However, exceptionally high-level aminoglycoside-resistance is achieved by the action of intrinsic and acquired 16S ribosomal RNA (rRNA) methyltransferase enzymes in aminoglycoside-producing and human pathogenic bacteria, respectively. These resistance determinants block drug binding by catalyzing the transfer of a methyl group from their cosubstrate S-adenosyl-l-methionine (SAM) to the base of a defined target RNA nucleotide within the ribosomal A-site. Here, we describe detailed structural and functional analyses of one of these enzymes, the kanamycin-resistance methyltransferase from Catenulisporales acidiphilia (‘CacKam’). CacKam has a SAM-binding core fold comprised of a seven-stranded β-sheet with a central topological switch point, characteristic of Class I methyltransferases.

We next exploited the altered crystal packing and constraints on the β6/7 linker in the CacKam-W203A crystal form to obtain a complex structure by soaking preformed crystals with SAM. In contrast to the apo structure of CacKam-W203A, SAM binding allowed the peptide backbone path of the β6/7 linker of one molecule (chain B) to be reliably modeled, albeit with significantly higher B-factors, in a conformation that is partially refolded on the SAM-binding pocket. The β6/7 linker of the second molecule in the asymmetric unit (chain A), however, remained disordered despite the presence of SAM in the ligand binding pocket. Interestingly, while the fully disordered linker of chain A is completely unrestrained by crystal packing, the β6/7 linker of chain B is adjacent to a symmetry related molecule. This molecular crowding in the crystal potentially mimics interaction with 30S and contributes to the observed closure of the linker exclusive to chain B. We conclude from these additional structures that cosubstrate binding alone likely does not drive complete reorganization of the β6/7 linker to a structure resembling that of NpmA or KamB. Instead this process must require direct interaction with the 30S substrate. However, significantly increased β6/7 linker B-factors in the CacKam-SAH complex, and the conversion of one CacKam-W203A β6/7 linker from fully disordered to partially closed in the apo form and SAM-bound forms, respectively, are both consistent with SAM binding being a prerequisite for β6/7 linker remodeling induced by interaction with 30S substrate.

>MHHHHHHASGLVPRGSHMTRTTALKVLAGKKLTDLDPDEWAKAQASAERILVDVGTGDARTAYRQAIAHPEWLVVGVDPAWQRMTETAVRAARKPAKGGAPNLVLVSSAIETVPAALHGVADEVMVLMPWGKLLRGVVLGEADVLSGLRAVAKPGAPLEISIGTSIWREPIPLEIRDLPELTPETVVSTGLTDRLAALGWQVADVRLVPHTDLDTISSSAARRLGSGATETVLHLRAVAVDPRDPVGTQHPAAESAQDTPEEPQRDV[2x]>MGNDISLIALLAFSTLLPFIIASGTCFVKFSIVFVMVRNALGLQQIPSNMTLNGVALLLSMFVMWPIMHDAYVYFEDEDVTFNDISSLSKHVDEGLDGYRDYLIKYSDRELVQFFENAQLKRQYGEETETVKRDKDEIEKPSIFALLPAYALSEIKSAFKIGFYLYLPFVVVDLVVSSVLLALGMMMMSPVTISTPIKLVLFVALDGWTLLSKGLILQYMDIAT[5x];> MFYALYFEIHHLVASAALGFARVAPIFFFLPFLNSGVLSGAPRNAIIILVALGVWPHALNEAPPFLSVAMIPLVLQEAAVGVMLGCLLSWPFWVMHALGCIIDNQRGATLSSSIDPANGIDTSEMANFLNMFAAVVYLQNGGLVTMVDVLNKSYQLCDPMNECTPSLPPLLTFINQVAQNALVLASPVVLVLLLSEVFLGLLSRFAPQMNAFAISLTVKSGIAVLIMLLYFSPVLPDNVLRLSFQATGLSSWFYERGATHVLE;>MDDLVFAGNKALYLVLILSGWPTIVATIIGLLVGLFQTVTQLQEQTLPFGIKLLGVCLCLFLLSGWYGEVLLSYGRQVIFLALAKG[4x];>MKTHILLARVLACAALVLVTPGYSSEKIPVTGSGFVAKDDSLRTFFDAMALQLKEPVIVSKMAARKKITGNFEFHDPNALLEKLSLQLGLIWYFDGQAIYIYDASEMRNAVVSLRNVSLNEFNNFLKRSGLYNKNYPLRGDNRKGTFYVSGPPVYVDMVVNAATMMDKQNDGIELGRQKIGVMRLNNTFVGDRTYNLRDQKMVIPGIATAIERLLQGEEQPLGNIVSSEPPAMPAFSANGEKGKAANYAGGMSLQEALKQNAAAGNIKIVAYPDTNSLLVKGTAEQVHFIEMLVKALDVAKRHVELSLWIVDLNKSDLERLGTSWSGSITIGDKLGVSLNQSSISTLDGSRFIAAVNALEEKKQATVVSRPVLLTQENVPAIFDNNRTFYTKLIGERNVALEHVTYGTMIRVLPRFSADGQIEMSLDIEDGNDKTPQSDTTTSVDALPEVGRTLISTIARVPHGKSLLVGGYTRDANTDTVQSIPFLGKLPLIGSLFRYSSKNKSNVVRVFMIEPKEIVDPLTPDASESVNNILKQSGAWSGDDKLQKWVRVYLDRGQEAIK[16x];>MIRRYLYTFLLVMTLAGCKDKDLLKGLDQEQANEVIAVLQMHNIEANKIDSGKLGYSITVAEPDFTAAVYWIKTYQLPPRPRVEIAQMFPADSLVSSPRAEKARLYSAIEQRLEQSLQTMEGVLSARVHISYDIDAGENGRPPKPVHLSALAVYERGSPLAHQISDIKRFLKNSFADVDYDNISVVLSERSDAQLQAPGTPVKRNSFATSWIVLIILLSVMSAGFGVWYYKNHYARNKKGITADDKAKSSNE[24x];>[24x]METSKEKTITSPGPYIVRLLNSSLNGCEFPLLTGRTLFVVGQSDALTASGQLPDIPADSFFIPLDHGGVNFEIQVDTDATEIILHELKEGNSESRSVQLNTPIQVGELLILIRPESEPWVPEQPEKLETSAKKNEPRFKNGIVAALAGFFILGIGTVGTLWILNSPQRQAAELDSLLGQEKERFQVLPGRDKMLYVAAQNERDTLWARQVLARGDYDKNARVI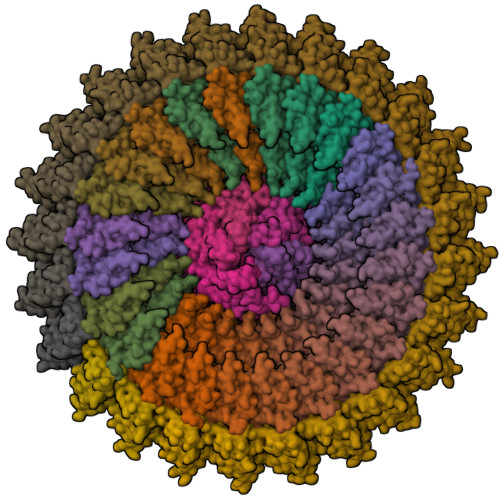NENEENKRISIWLDTYYPQLAYYRIHFDEPRKPVFWLSRQRNTMSKKELEVLSQKLRALMPYADSVNITLMDDVTAAGQAEAGLKQQALPYSRRNHKGGVTFVIQGALDDVEILRARQFVDSYYRTWGGRYVQFAIELKDDWLKGRSFQYGAEGYIKMSPGHWYFPSPL> MKIAGIDEAGRGPVIGPMVIAAVVVDENSLPKLEELKVRDSKKLTPKRREKLFNEILGVLDDYVILELPPDVIGSREGTLNEFEVENFAKALNSLKVKPDVIYADAADVDEERFARELGERLNFEAEVVAKHKADDIFPVVSAASILAKVTRDRAVEKLKEEYGEIGSGY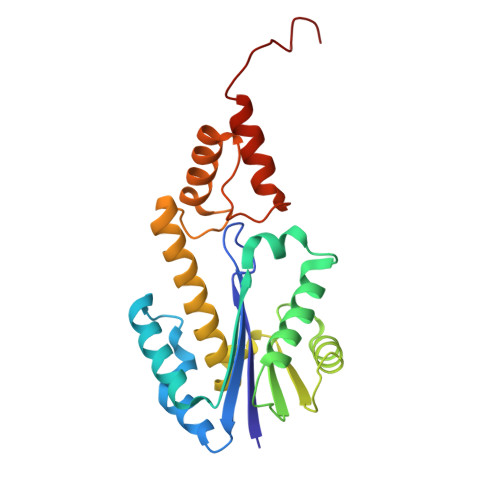PSDPRTRAFLENYYREHGEFPPIVRKGWKTLKKIAEKVESEKTQDMINKST> AKCVSYGVAQIKAPALHSQGYTGSNVKVAVLDSGIDSSHPDLNVAGGASFVPSETNPFQDNNSHGTHVAGTVLAVAPSASLYAVKVLGADGSGQYSWVINGIEWAIANNMDVINMSLGGPSGSAALKAAVDKAVASGVVVVAAAGNSGTSGSSSTVSYPAKYPSVIAVGAVDSSNQRAPFSSVGPELDVMAPGVSICSTLPGGKYGAHS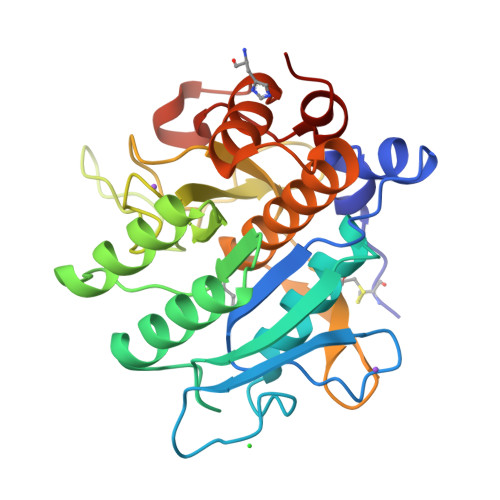GTCPASNHVAGAAALILSKHPNWTNTQVRSSLENTATKLGDSFYYGKGLINVEAAAQHHHHHH>MGHHHHHHMATEKKEADNVAISVDVLTKYKTAAQISEKVLAEVSKLCVPGAKIIDICEQGDKLMEEELSKVYRDKKTNKGFSHPTTVSPAAFITPYTPLRSDEKEAATEIQPGEPIKIQLGAQIDGYGTIVCDTIVAKNANDPDVIEGRQADLFLATYYANEVLLRLMVPPGLLATGTDEEKAKAAAVKPPSQAKISSLLEKVAKAYDCNIIESTTSWLFDKNEIEGKKKIILSPGENIKGEGVPEVGDVWGVEVGCSLGSGKVKQFEQRATLHRRTNNTYALKRPTSRKIYSEVQKKFGTFPFSLRQLEDERDAKSGVIECVRGGVFRQYEVTGDKDNAPVCRLLTTIAITKNGITRIGGPPAWDLSKFKTDK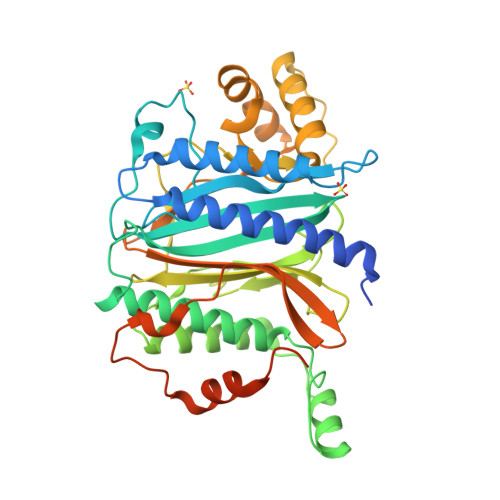KIEDEEILKILEQPLSKNAGKNKNKKKKKKAKKAAAKPDEGEEESSDEE[4x]> MGSSHHHHHHSSGRENLYFQGHMNGDQNSDVYAQEKQDFVQHFSQIVRVLTEDEMGHPEIGDAIARLKEVLEYNAIGGKYNRGLTVVVAFRELVEPRKQDADSLQRAWTVGWCVELLQAFFLVADDIMDSSLTRRGQICWYQKPGVGLDAINDANLLEACIYRLLKLYCREQPYYLNLIELFLQSSYQTEIGQTLDLLTAPQGNVDLVRFTEKRYKSIVKYKTAFYSFYLPIAAAMYMAGIDGEKEHANAKKILLEMGEFFQIQDDYLDLFGDPSVTGKIGTDIQDNKCSWLVVQCLQRATPEQYQILKENYGQKEAEKVARVKALYEELDLPAVFLQYEEDSYSHIMALIEQYAAPLPPAVFLGLARKIYKRRK

At the first branching point in this pathway lies farnesyl pyrophosphate synthase (FPPS). FPPS catalyses the sequential condensation of dimethylallyl pyrophosphate (DMAPP) with isopentenyl pyrophosphate (IPP) and the resulting geranyl pyrophosphate (GPP) with another unit of IPP, eventually producing the 15-carbon isoprenoid farnesyl pyrophosphate (FPP). The binding of an allylic substrate induces an open-to-closed conformational change in the enzyme, which reshapes its active site cleft and thereby fully forms the IPP-binding site. Inhibition of the enzyme has been well established as the mechanism of action of nitrogen-containing bisphosphonates (N-BPs), blockbuster drugs that are widely used against bone resorption disorders.

Human FPPS was crystalized in the presence of FPP, and its X-ray structure was determined at 1.9 Å resolution (Rwork/Rfree=0.172/0.211). Binding of the product at the previously speculated allosteric pocket was unambiguous based on the electron density and anomalous signals. The α-phosphate of FPP occupies the entrance of this pocket, engaged in a H-bond with Asn59 and a quadrupole–charge interaction with Phe239. The β-phosphate sits at the edge of the IPP-binding site, forming salt bridges with Lys57 and Arg60; these residues interact with the α-phosphate of IPP when IPP is bound. The tail of FPP extends deep into the allosteric pocket, making tight van der Waals contacts with the protein surface. Furthermore, FPP binding entails an induced-fit conformational change that has not been observed with other allosteric ligands. The key residues include Tyr10, which swings away from αC to accommodate the tail end of FPP. Essentially, the conformational change expands the allosteric pocket and reshapes its surface for better steric complementarity with the long hydrocarbon tail of FPP. With FPP bound in the allosteric pocket, the enzyme adopts the open conformational state. Therefore, allosterically bound FPP can be considered as a molecular wedge that prohibits this conformational transition via steric hindrance.>[4x]MEISQPSIGIFYISKVLALAPYATVRNSKGRVEIGRSWLFTVYSATLTVVMVFLTYRGLLFDANSEIPVRMKSATSKVVTALDVSVVVMAIVSGVYCGLFSLNDTLELNDRLNKIDNTLNAYNNFRRDRWRALGMAAVSLLAISILVGLDVGTWMRIAQDMNIAQSDTELNVHWYIPFYSLYFILTGLQVNIANTAYGLGRRFGRLNRMLSSSFLAENNATSA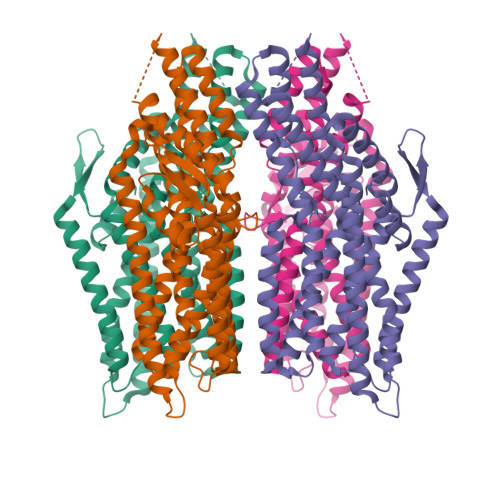IKPQKVSTVKNVSVNRPAMPSALHASLTKLNGETLPSEAAAKNKGLLLKSLADSHESLGKCVHLLSNSFGIAVLFILVSCLLHLVATAYFLFLELLSKRDNGYLWVQMLWICFHFLRLLMVVEPCHLAARESRKTIQIVCEIERKVHEPILAEAVKKFWQQLLVVDADFSACGLCRVNRTILTSFASAIATYLVALIQFQRTNGLEGGSSGGWSHPQFEK> VTNVGEDGEPGETEPRHALSPVDMHVHTDVSFLLDRFFDVETLELSNLTGSPATHVLDPFGSTAQLAWARLLNTCTYFFSDLELSIQFKFTTTPSSVGEGFVWVKWFPVGAPTKTTDAWQLEGGGNSVRIQQLAVAGMSPTVVFKIAGSRSQACGFSVPYTSMWRVVPVFYNGWGAPTKEKATYNWLPGAHFGSILLTSDAHDKGGCYLRYRFPRANMYCPRPIPPAFTRPADKTRHKFPTNINKQ;> DKKTEETTNIEDRIETTVVGATIINSQGSVGTTYCYSKPDGRPPSTVSDPVTRLGPTLSRHYTFKVGEWPHSQSHGHAWICPLPSDKLKKMGSFHEVVKAHHLVKNGWDVVVQVNASFAHSGALCVAAVPEYEHTHEKALKWSELEEPAYTYQQLSVFPHQLLNLRTNSSVHLVMPYIGPGPTTNLTLHNPWTIVILILSELTGPGQTVPVTMSVAPIDAMVNGPLPNPE;> APIRVVSVPESDSFMSSVPDNSTPLYPKVVVPPRQVPGRFTNFIDVAKQTYSFCSISGKPYFEVTNTSGDEPLFQMDVSLSAAELHGTYVASLSSFFAQYRGSLNFNFIFTGAAATKAKFLVAFVPPHSAAPKTRDEAMACIHAVWDVGLNSAFSFNVPYSSPADFMAVYSAEATVVNVSGWLQVYALTALTSTDIAVNSKGRVLVAVSAGPDFSLRHPVDLPDKQ;> GAGTSTPTTGNQNMSGNSGSIVQNFYMQQYQNSIDADLGDNVISPEGQGSNTSSSTSSSQSSGLGGWFSSLLNLGTKLLA

Equine rhinitis A virus (ERAV) shares physicochemical properties such as buoyant density, base composition and acid lability with foot-and-mouth-disease virus (FMDV). The mature capsid comprises 60 copies of each of four proteins: VP1-4 (with molecular weights of 25, 25, 22 and 11 kDa respectively for ERAV). VP1-3 are composed of eight-stranded β-sandwiches, with strands denoted CHEF and BIDG respectively on the two sheets, which form a pseudo T = 3 icosahedral lattice with the CHEF sheet exposed on the capsid surface and BIDG to the interior. To investigate how similar ERAV and FMDV are in terms of structure and to probe further the cell entry mechanism for aphthoviruses we have determined crystal structures of ERAV at two different pHs, using highly optimised methods since the yield of purified virus was very low.

Since the pH of crystallization liquor for this structure was 4.6 (tests confirmed that the virus solution did not significantly perturb this) we might have expected to see dissociated pentamers rather then intact particles. However, the structure was clearly of an intact particle, although the disorder of certain features on the inside of the capsid prompted us to try to solve the structure of the virus at physiological pH. There are however significant rearrangements, and an overall loss of order, in several internal loops. Thus the entire first 31 residues of VP2 cannot be clearly defined, including the hairpin structure which is generally well conserved and is a crucial element in stabilizing the pentamer interface. The VP1 N-terminus rearranges to form a loop close to the pentamer interface underlying VP3 and adjacent to the site of residues 78–88 of VP4 in FMDV. It thus occupies the position that would otherwise be occupied by the VP2 hairpin from an adjacent pentamer and replaces some of the stabilizing interactions at the pentamer interface, however overall the inter-pentamer interface between VP2 and VP3 is weakened. In contrast there do not appear to be any significant rearrangements on the capsid exterior surface, only slight deviations in loop conformations and side-chain orientations. In contrast the low pH ERAV structure shows weakened interactions at the pentamer interface, with no ordered electron density for the VP2 N-terminal hairpin, which is partly replaced by the N-terminus of VP1 from an adjacent pentamer which contributes a few stabilizing interactions, consistent with a particle en-route to dissociation. This structure likely corresponds to the transient empty particle seen in the biochemical analyses but both experiments are suggestive of disassembly intermediates not previously reported.>[4x]MAKTQAEINKRLDAYAKGTVDSPYRVKKATSYDPSFGVMEAGAIDADGYYHAQCQDLITDY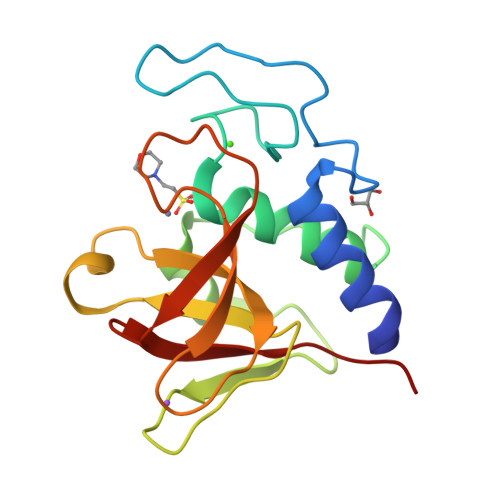VLWLTDNKVRTWGNAKDQIKQSYGTGFKIHENKPSTVPKKGWIAVFTSGSYEQWGHIGIVYDGGNTSTFTILEQNWNGYANKKPTKRVDNYYGLTHFIEIPVKA> SEKPRCAGCDELIFSNEYTQAENQNWHLKHFCCFDCDSILAGEIYVMVNDKPVCKPCYVKNHAVVCQGCHNAIDPEVQRVTYNNFSWHASTEC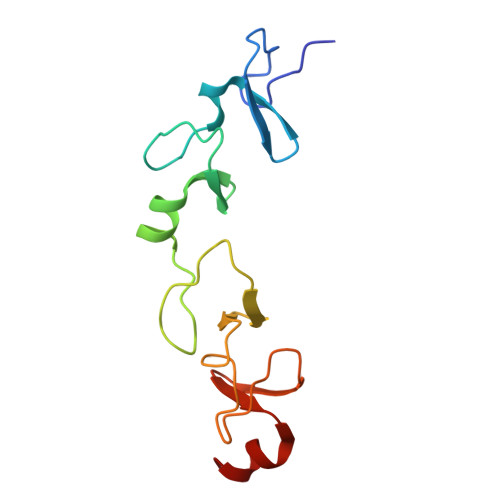FLCSCCSKCLIGQKFMPVEGMVFCSVECKKRMS> GLTPEQKQKKAALSASEGEEVPQDKAPSHVPFLLIGGGTAAFAAARSIRARDPGARVLIVSEDPELPYMRPPLSKELWFSDDPNVTKTLRFKQWNGKERSIYFQPPSFYVSAQDLPHIENGGVAVLTGKKVVQLDVRDNMVKLNDGSQITYEKCLIATGGTPRSLSAIDRAGAEVKSRTTLFRKIGDFRSLEKISREVKSITIIGEGFLGSELACALGRKARALGTEVIQLFPEKGNMGKILPEYLSNWTMEKVRREGVKVMPNAIVQSVGVSSGKLLIKLKDGRKVETDHIVAAVGLEPNVELAKTGGLEIDSDFGGFRVNAELQARSNIWVAGDAACFYDIKLGRRRVEHHDHAVVSGRLAGENMTGAAKPYWHQSMFWSDLGPDVGYEAIGLVDSSLPTVGVFAKATAQDNPKSATEQSGTGIRSESETESRASEITIPPSTPAVPQAPVQGEDYGKGVIFYLRDKVVVGIVLWNIFNRMPIARKIIKDGEQHEDLNEVAKLFNIHEDLVP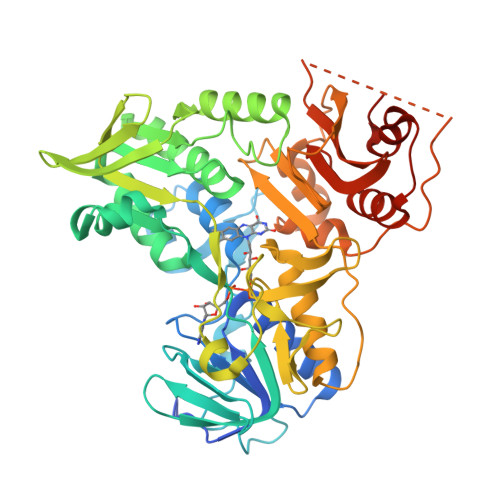R> GSGSGSGSGSGSGSGSGSMAEPASVAAESLAGSRARAARTVLGQVVLPGEELLLPEQEDAEGPGGAVERPLSLNARACSRVRVVCGPGLRRCGDRLLVTKCGRLRH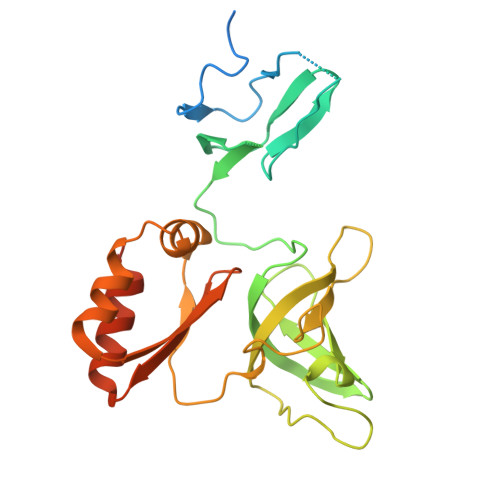KEPGSGSGGGVYWVDSQQKRYVPVKGDHVIGIVTAKSGDIFKVDVGGSEPASLSYLSFEGATKRNRPNVQVGDLIYGQFVVANKDMEPEMVCIDSCGRANGMGVIGQDGLLFKVTLGLIRKLLAPDCEIIQEVGKLYPLEIVFGMNGRIWVKAKTIQQTLILANILEACEHMTSDQRKQIFSRLAES> MNVRVLVVEDERDLADLITEALKKEMFTVDVCYDGEEGMYMALNEPFDVVILDIMLPVHDGWEILKSMRESGVNTPVLMLTALSDVEYRVKGLNMGADDYLPKPFDLRELIARVRALIRRKSESKSTKLVCGDLILDTATKKA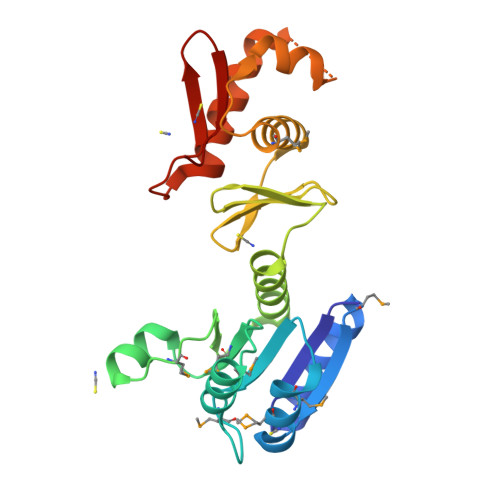YRGSKEIDLTKKEYQILEYLVMNKNRVVTKEELQEHLWSFDDEVFSDVLRSHIKNLRKKVDKGFKKKIIHTVRGIGYVARDE> LKESPSGYLRSGEGDTGCGELVWVGEPLTLRTAETITGKYGVWMRDPKPTYPYTQETTWRIDTVGTDVRQVFEYDLISQFMQGYPSKVHILPRPLESTGAVVYSGSLYFQGAESRTVIRYELNTETVKAEKEIPGAGYHGQFPYSWGGYTDIDLAVDEAGLWVIYSTDEAKGAIVLSKLNPENLELEQTWETNIRKQSVANAFIICGTLYTVSSYTSADATVNFAYDTGTGISKTLTIPFKNRYKYSSMINYNPLEKKLFAWDNLNMVTYDIKLS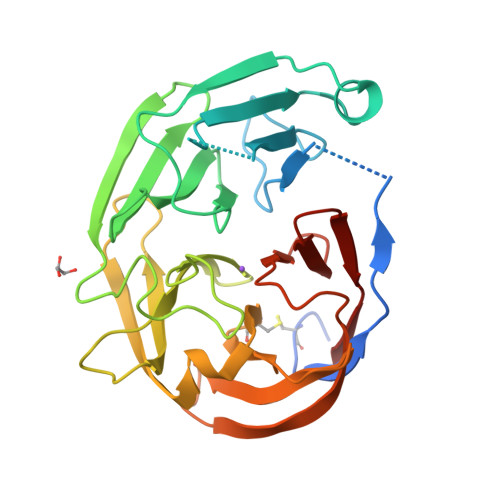KM>MSRILLSSLLAAGLFCSLPASAATGCMLFADGSGKPFSAQGDCASQLPPASTFKIPLALMGYDSGFLVDEQLPALPFKAGDPDFLPEWKQTTTPSRWMTYSVIWYSQRLTEWLGAARFQQYVDRFDYGNRDLSGNPGKHDGLTQAWLSSSLAISPQEQARFLGKLVSGKLPVSAQTLQHTANILRQPDIDGWQIHGKTGTGYPKLLDGSLDRDQQIGWFVGWASKQDQKLIFVHTVIQKPGKQFASLRAREEVFAALPEQLKKLVEHHHHH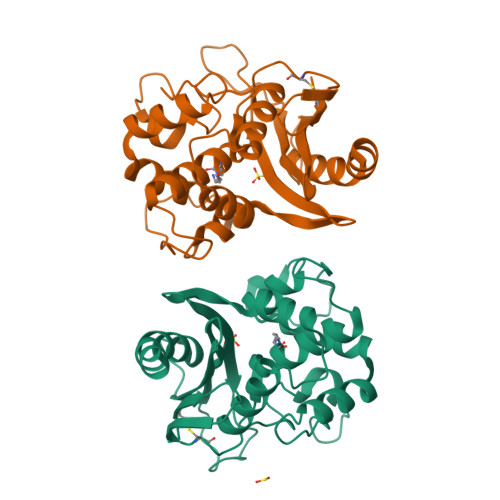HHH[2x]> EQSSSEIKIVRDEYGMPHIYANDTWHLFYGYGYVVAQDRLFQMEMARRSTQGTVAEVLGKDFVKFDKDIRRNYWPDAIRAQIAALSPEDMSILQGYADGMNAWIDKVNTNPETLLPKQFNTFGFTPKRWEPFDVAMIFVGTMANRFSDSTSEIDNLALLTALKDKYGVSQGMAVFNQLKWLVNPSAPTTIAVQESNYPLKFNQQNSQTA;> SNMWVIGKSKAQDAKAIMVNGPQFGWYAPAYTYGIGLHGAGYDVTGNTPFAYPGLVFGHNGVISWGSTAGFGDDVDIFAERLSAEKP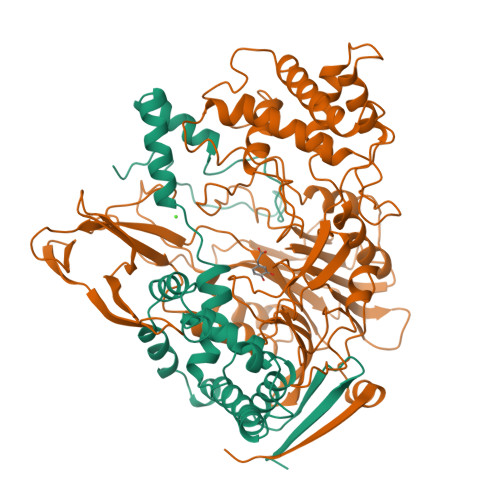GYYLHNGKWVKMLSREETITVKNGQAETFTVWRTVHGNILQTDQTTQTAYAKSRAWDGKEVASLLAWTHQMKAKNWQQWTQQAAKQALTINWYYADVNGNIGYVHTGAYPDRQSGHDPRLPVPGTGKWDWKGLLPFEMNPKVYNPQSGYIANWNNSPQKDYPASDLFAFLWGGADRVTEIDRLLEQKPRLTADQAWDVIRQTSRQDLNLRLFLPTLQAATSGLTQSDPRRQLVETLTRWDGINLLNDDGKTWQQPGSAILNVWLTSMLKRTVVAAVPMPFDKWYSASGYETTQDGPTGSLNISVGAKILYEAVQGDKSPIPQAVDLFAGKPQQEVVLAALEDTWETLSKRYGNNVSNWKTPAMALTFRANNFFGVPQAAAEETRHQAEYQNRGTENDMIVFSPTTSDRPVLAWDVVAPGQSGFIAPDGTVDKHYEDQLKMYENFGRKSLWLTKQDVEAHKESQEVLHVQR> ANFVTDSEVTKLKWSKAPCRFCGTGCGVTVAVKDNKVVATQGDPQAEVNKG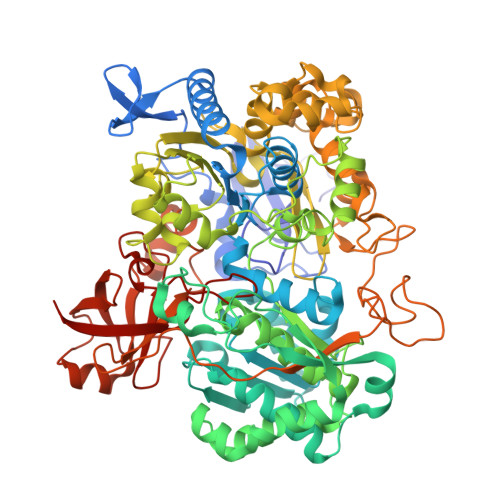LNCVKGYFLSKIMYGQDRLTRPLMRMKNGKYDKNGDFAPVTWDQAFDEMERQFKRVLKEKGPTAVGMFGSGQWTVWEGYAAAKLYKAGFRSNNIDPNARHCMASAAAGFMRTFGMDEPMGCYDDFEAADAFVLWGSNMAEMHPILWTRVTDRRLSHPKTRVVVLSTFTHRCFDLADIGIIFKPQTDLAMLNYIANYIIRNNKVNKDFVNKHTVFKEGVTDIGYGLRPDHPLQKAAKNASDPGAAKVITFDEFAKFVSKYDADYVSKLSAVPKAKLDQLAELYADPNIKVMSLWTMGFNQHTRGTWANNMVYNLHLLTGKIATPGNSPFSLTGQPSACGTAREVGTFSHRLPADMVVTNPKHREEAERIWKLPPGTIPDKPGYDAVLQNRMLKDGKLNAYWVQVNNNMQAAANLMEEGLPGYRNPANFIVVSDAYPTVTALAADLVLPSAMWVEKEGAYGNAERRTQFWHQLVDAPGEARSDLWQLVEFAKRFKVEEVWPPELIAKKPEYKGKTLYDVLYRNGQVDKFPLKDVNAEYHNAEAKAFGFYLQKGLFEEYATFGRGHGHDLAPFDAYHEARGLRWPVVNGKETRWRYREGSDPYVKAGTGFQFYGNPDGKAVIFALPYEPPAESPDKEYPYWLVTGRVLEHWHSGSMTRRVPELYRSFPNAVVFMHPEDAKALGLRRGVEVEVVSRRGRMRSRIETRGRDAPPRGLVFVPWFDASQLINKVTLDATCPISLQTDFKKCAVKIVKV(1S,3S,4S,5S)-7,7-dichloro-3-methoxy-2-thiabicyclo[3.2.0]heptan-6-one-4-carboxylic acid | 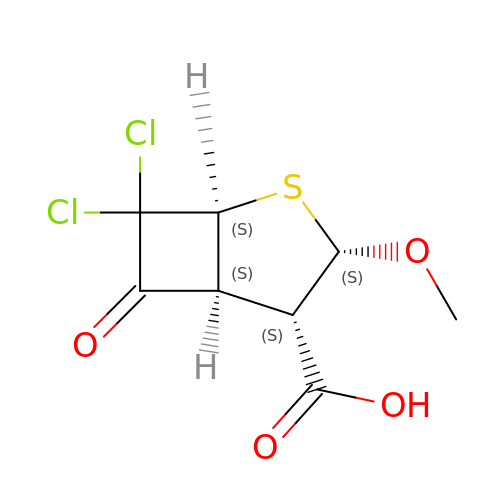C8 H8 Cl2 O4 S | PELFTKQNZKVHIO-NXTKUWPGSA-N N-[4-(1-ALLYL-3-BUTYL-2,6-DIOXO-2,3,6,7-TETRAHYDRO-1H-PURIN-8-YLMETHYL)-PHENYL]-ACETAMIDE | C21 H25 N5 O3 | 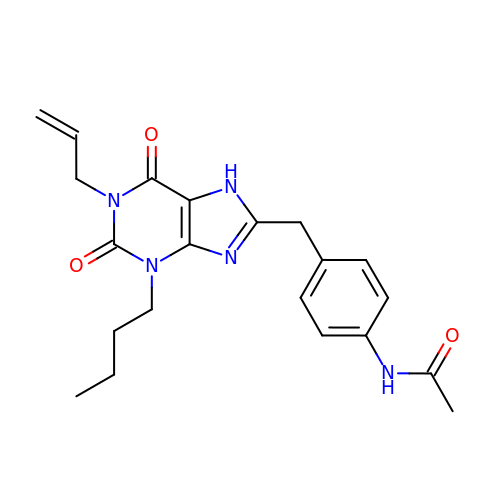XFOWZKUTPKXWIE-UHFFFAOYSA-N> VVSKLFFSWTRPILRKGYRQRLELSDIYQIPSVDSADNLSEKLEREWDRELASKKNPKLINALRRCFFWRFMFYGIFLYLGEVTKAVQPLLLGRIIASYDPDNKEERSIAIYLGIGLCLLFIVRTLLLHPAIFGLHHIGMQMRIAMFSLIYKKTLKLSSRVLDKISIGQLVSLLSNNLNKFDEGLALAHFVWIAPLQVALLMGLIWELLQASAFCGLGFLIVLALFQAGLGRMMMKYRDQRAGKISERLVITSEMIENIQSVKAYCWEEAMEKMIENLRQTELKLTRKAAYVRYFNSSAFFFSGFFVVFLSVLPYALIKGIILRKIFTTISFCIVLRMAVTRQFPWAVQTWYDSLGAINKIQDFLQKQEYKTLEYNLTTTEVVMENVTAFWEEGFGELFEKAKQNNNNRKTSNGDDSLFFSNFSLLGTPVLKDINFKIERGQLLAVAGSTGAGKTSLLMVIMGELEPSEGKIKHSGRISFCPQFPWIMPGTIKENIIFGVSYDEYRYRSVIKACQLEEDISKFPEKDNTVLGEGGITLSGGQRAKISLARAVYKDADLYLLDSPFGYLDVLTEKEIFESCVCKLMANKTRILVTSKMEHLKKADKILILHEGSSYFYGTFSELQNLQPDFSSKLMGCDSFDQFSAERRNSILTETLHRFSLEGDAPVSWTETKKQSFKQTGEFGEKRKNSILNPINSIRKFSIVQKTPLQMNGIEEDSDEPLERRLSLVPDSEQGEAILPRISVISTGPTLQARRRQSVLNLMTHSVNQGQNIHRKTTASTRKVSLAPQANLTELDIYSRRLSQETGLEISEEINEEDLKECFFDDMESIPAVTTWNTYLRYITVHKSLIFVLIWCLVIFLAEVAASLVVLWLLGNTPLQDKGNSTHSRNNSYAVIITSTSSYYVFYIYVGVADTLLAMGFFRGLPLVHTLITVSKILHHKMLHSVLQAPMSTLNTLKAGGILNRFSKDIAILDDLLPLTIFDFIQLLLIVIGAIAVVAVLQPYIFVATVPVIVAFIMLRAYFLQTSQQLKQLESEGRSPIFTHLVTSLKGLWTLRAFGRQPYFETLFHKALNLHTANWFLYLSTLRWFQMRIEMIFVIFFIAVTFISILTTGEGEGRVGIILTLAMNIMSTLQWAVNSSIDVDSLMRSVSRVFKFIDMPTEGKPTKSTKPYKNGQLSKVMIIENSHVKKDDIWPSGGQMTVKDLTAKYTEGGNAILENISFSISPGQRVGLLGRTGSGKSTLLSAFLRLLNTEGEIQIDGVSWDSITLQQWRKAFGVIPQKVFIFSGTFRKNLDPYEQWSDQEIWKVADEVGLRSVIEQFPGKLDFVLVDGGCVLSHGHKQLMCLARSVLSKAKILLLDQPSAHLDPVTYQIIRRTLKQAFADCTVILCEHRIEAMLECQQFLVIEENKVRQYDSIQKLL

In the human body, the chloride channel Cystic Fibrosis Transmembrane conductance Regulator (CFTR) mediates chloride transport across the cell membrane in multiple epithelial-lining organs, including intestines, biliary ducts, pancreas ducts, respiratory airways, and sweat ducts. Topological analysis of CFTR places it in the ATP-binding Cassette (ABC) transporter family, which harnesses the energy from ATP hydrolysis to move substrates across cell membranes. Structurally, ABC proteins possess two transmembrane domains (TMDs) forming the substrate translocation pathway and two cytosolic nucleotide-binding domains (NBDs) that recruit and hydrolyze ATP as the energy source. Once the R domain is phosphorylated, ATP-binding induced NBD dimerization and subsequent hydrolysis of ATP in site 2 are coupled to the opening and closing of the CFTR pore, respectively.

The current study reported two cryo-EM structures of E1371Q-CFTR proteins produced by a lentiviral expression system. The E1371Q-CFTR proteins so produced show highly uniform conformations owing to the E-to-Q mutation abolishing ATP hydrolysis at CFTR’s site 222,68. The yield of the E1371Q-CFTR mutant is high, ensuring that the sample can be effectively concentrated for cryo-grids freezing and that abundant protein particles can be imaged for cryo-EM structure determination. The sharp and symmetric elution peak of E1371Q-CFTR proteins from size exclusion chromatography (SEC) indicates that the sample has high purity and homogeneity, both of which are characteristics ideal for cryo-EM studies. The negative staining images of E1371Q-CFTR, in which individual intact CFTR protein molecules can be readily discerned, show that the proteins are mono-dispersed and not prone to aggregate at room temperature. Upon deposition on cryo-grids, the mono-dispersity of E1371Q-CFTR protein particles is maintained, which facilitates later particle picking and processing. With this high-quality sample, the electron density map of E1371Q-CFTR was determined at an overall resolution of 3.4 Å where densities of the side chains for most amino acids are clearly defined. Our cryo-EM analysis of the E1371Q-CFTR mutant reached an overall resolution of 3.4 Å and revealed a conformation closely resembling the previous structure obtained using the BacMam system, affirming the compatibility of the lentiviral expression system with the BacMam system in producing high-quality CFTR proteins for cryo-EM studies. Thus, the mutations introduced to stabilize the CFTR protein do not disturb the overall structure of the E1371Q-CFTR protein. The fact that the phosphorylated, ATP-bound E1371Q-CFTR conformation is well conserved regardless of the presence of various CFTR potentiators and correctors suggests that this is a stable conformation representing an activated CFTR channel.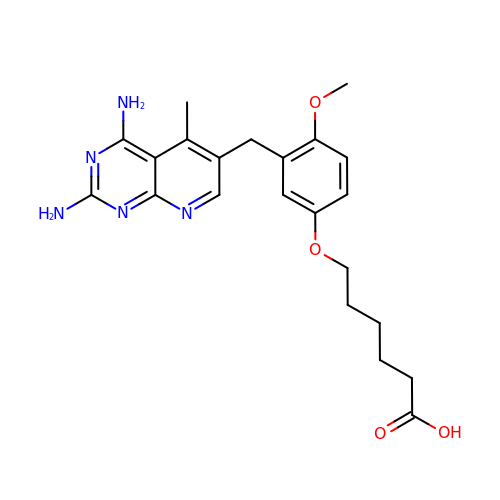6-{3-[(2,4-diamino-5-methylpyrido[2,3-d]pyrimidin-6-yl)methyl]-4-methoxyphenoxy}hexanoic acid | C22 H27 N5 O4 | MMMXXNOXIQPQHJ-UHFFFAOYSA-N> EVDKRREINNEHPLLMMPLYANGEEFNQGKYTFWGGDTLTGKWENIPDDLKPYTVIQLHPDDLPKRDGAARDFYEHMLEEAAKYVNPKTGKNEPIPVILTVYTAGNMPYYTSAHWLSTSWIDKMYQKYPNLHGIFSTASYWIWANDIENKAADYLKVSAKNGGYFIWAEQNSGSAIEKAFGKNGKIAFQKSVDKYWKNLIFMFKNTPAAEGNDSTTESYMKGLWLSNHTYQWGGLMDTWKWYETGKWKLFASGNIGKSQGDRQWLTEPESMLGEEALGVYLNGGVVYNFEHPAYTYGVNNKESLLFSEVIKEFFRYVIAHPAPSKEKVLEDTKVFIHGDYSNKGNGKFFVNVNTDREQTPLYMTGRYNVIP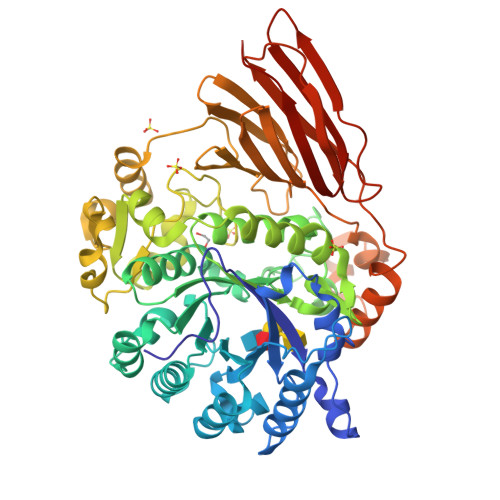AIPGVLKTDKLKESVSSSRIQIKEITSPEFSSTQARKEYLNKLYPMNYEGDIFAQKLDNRWFVYNYKVNENVKQTGKLKFNSLEMNVEFEPHTYGIFERISNGLKVNLNNFRTNKDSLWSNAQDANQAKKLPQLTKKGAIKWIEEHYIKDTQFGEKRVTKIVLRGIDKLPTIHSLSGTNNSYDQPSLNFDQKNHMVTITINSNGNLEFELHFLEHPPPPPLRSGC> GELDELVYL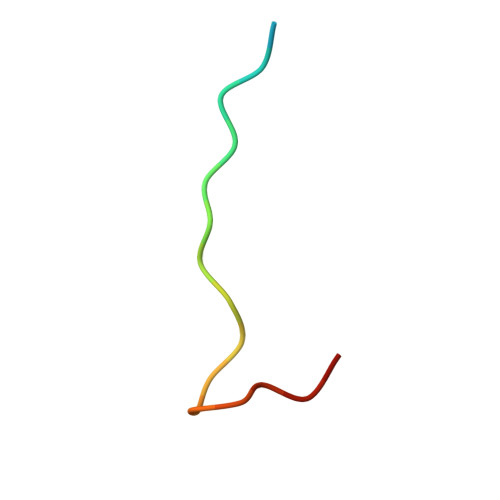LDGPGYDPIHS>[2x]TTGHSYEKYNNWETIEAWTKQVTSENPDLISRTAIGTTFLGNNIYLLKVGKPGPNKPAIFMDCGFHAREWISHAFCQWFVREAVLTYGYESHMTEFLNKLDFYVLPVLNIDGYIYTWTKNRMWRKTRSTNAGTTCIGTDPNRNFDAGWCTTGASTDPCDETYCG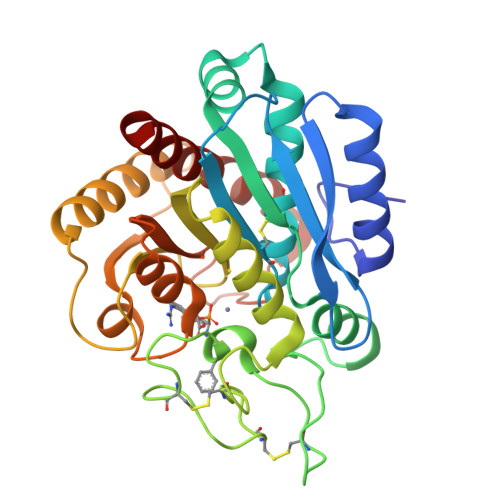SAAESEKETKALADFIRNNLSSIKAYLTIHSYSQMILYPYSYDYKLPENNAELNNLAKAAVKELATLYGTKYTYGPGATTIYPAAGGSDDWAYDQGIKYSFTFELRDKGRYGFILPESQIQATCEETMLAIKYVTNYVLGHL methyl [(6S)-4-(4-chlorophenyl)-2,3,9-trimethyl-6H-thieno[3,2-f][1,2,4]triazolo[4,3-a][1,4]diazepin-6-yl]acetate 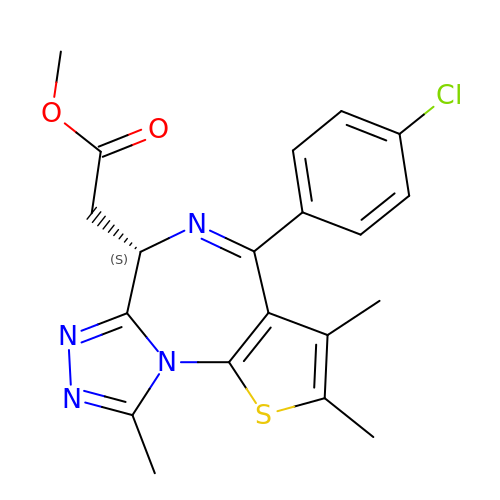| C20 H19 Cl N4 O2 S | GGRCIHACOIMRKY-HNNXBMFYSA-N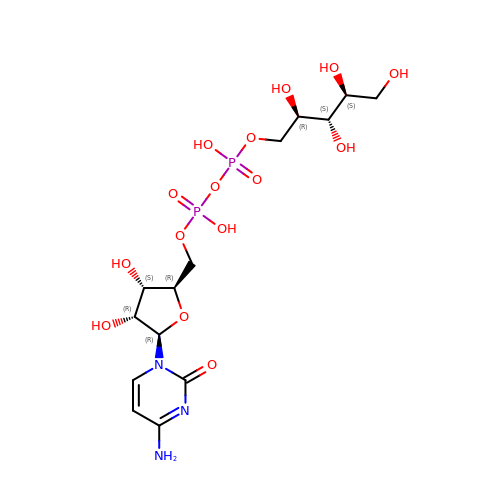CDP-ribitol | C14 H25 N3 O15 P2 | DPJKHFICSGCNIR-HRENORGGSA-N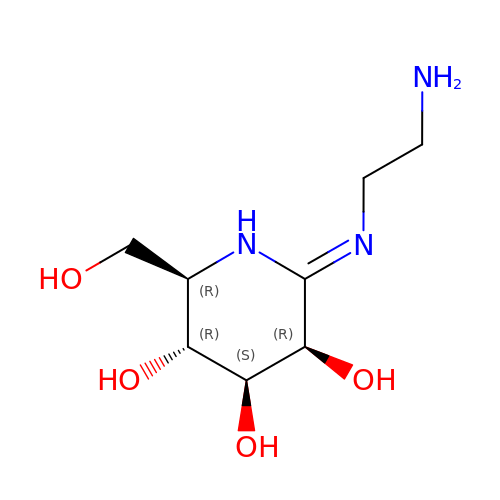(2Z,3R,4S,5R,6R)-2-[(2-aminoethyl)imino]-6-(hydroxymethyl)piperidine-3,4,5-triol | C8 H17 N3 O4 | ZLIQDFHJGBHZAQ-JWXFUTCRSA-N> MGQKIGILGAMREEITPILELFGVDFEEIPLGGNVFHKGVYHNKEIIVAYSKIGKVHSTLTTTSMILAFGVQKVLFSGVAGSLVKDLKINDLLVATQLVQHDVDLSAFDHPLGFIPESAIFIETSGSLNALAKKIANEQHIALKEGVIASGDQFVHSKERKEFLVSEFKASAVEMEGASVAFVCQKFGV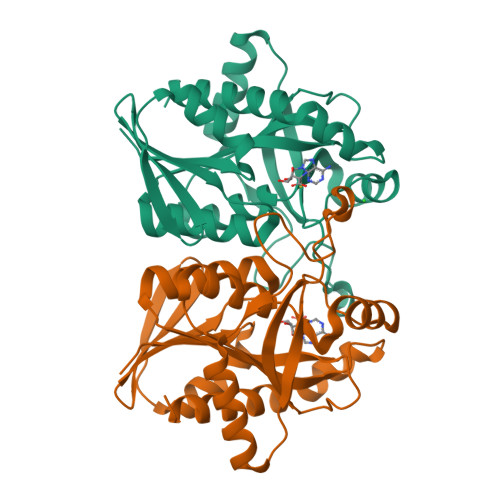PCCVLRSISNNADEKAGMSFDEFLEKSAHTSAKFLKSMVDEL> VVEAVENAVARVADTISSGPSNSQAVPALTAVETGHTSQVTPSDTIQTRHVRNYHSRSESSIENFLCRSACVYMGEYHTTNTDTSKLFASWTINARRMVQMRRKLELFTYVRFDMEVTFVITSKQDQGTQLGQDMPPLTHQIMYIPPGGPIPKSVTDYTWQTSTNPSIFWTEGNAPPRMSIPFISIGNAYSNFYDGWSHFSQNGVYGYNTLNHMGQIYVRHVNGSSPLPMTSTVRMYFKPKHVKVWVPRPPRLCQYKNASTVNFTPTNITEKRQSINYIPETVKP;> DRVRSITLGNSTITTQESANVVVAYGRWPEYLKDNEATAEDQPTQPDVATCRFYTLESVTWERDSPGWWWKFPDALK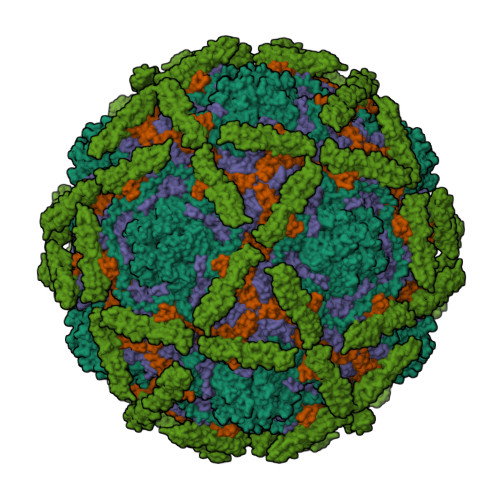DMGLFGQNMYYHYLGRAGYTIHVQCNASKFHQGCLMVVCVPEAEMGCSQVDGTVNEHSLSEGETAKKFASTSTNGTNTVQSIVTNAGMGVGVGNLTIFPHQWINLRTNNCATIVMPYINNVPMDNMFRHHNFTLMIIPFVPLDYSSDSSTYVPITVTVAPMCAEYNGLRLATSL;> GLPVMNTPGSNQFLTSDDFQSPSAMPQFDVTPELNIPGEVQNLMEIAEVDSVVPVNNVEGKLDTMEIYRIPVQSGNHQSSQVFGFQVQPGLDNVFKHTLLGEILNYYAHWSGSIKLTFVFCGSAMATGKFLLAYAPPGANAPKSRKDAMLGTHIIWDVGLQSSCVLCIPWISQTHYRLVQQDEYTSAGNVTCWYQTGIVVPAGTPTSCSIMCFVSACNDFSVRLLKDTPFIEQSALLQ;> MGAQVSTQKTGAHETGLNASGRSIIHYTNINYYKDAASNSANRQDFSQDPGKFTEPVKDIMVKSLPALN;> KSCPNPGEIRNGQIDVPGGILFGATISFSCNTGYKLFGSTSSFCLISGSSVQWSDPLPECREIYCPAPPQIDNGIIQGERDHYGYRQSVTYACNKGFTMIGEHSIYCTVNNDEGEWSGPPPECRG>MIEKFIMAGPTALHVCDSQKGDKCVVLLHGYLESMLVWEDFVPFLYKELRVVTLDLPGHGISVVTGEEHSMEFLAD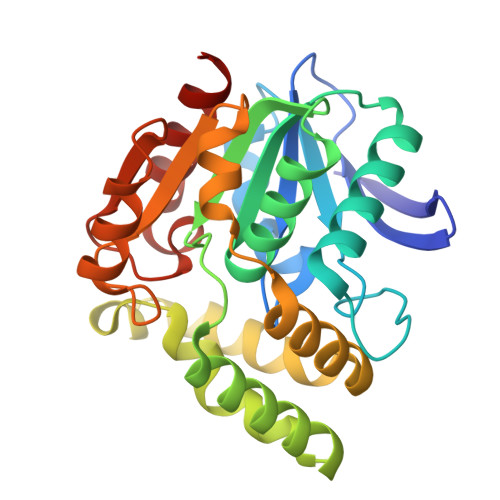TVADALRALGIPRCTLVGHSMGGYVALAFCERHPDMLNGVVLLSSTPNADTPEKSENRRREIALVKAGKKDALARVAPEAGFAEDNRTRMKDYIEDLTEQVAVTEDEGIVALLNGMIARKDQNEMLRASKVPQLFILGRKDNYIPVEAAEKMVKEHLQARVVWLENSGHMGFLEEPETTARAILDFVNGK[4x]N-benzyl-1-{3-[(2-chloro-5-{5-(methylsulfonyl)-1-[3-(morpholin-4-yl)propyl]-4,5,6,7-tetrahydro-1H-pyrazolo[4,3-c]pyridin-3-yl}phenyl)ethynyl]phenyl}methanamine | C36 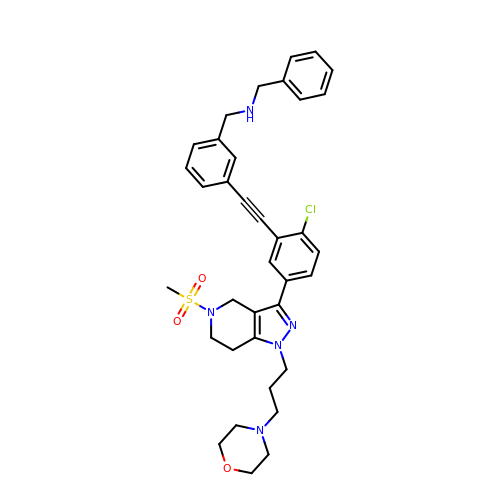H40 Cl N5 O3 S | LIGRCXVOYJUELL-UHFFFAOYSA-N>[2x]AGHMKEIKEITKKDVQDAEIYLYGSVVEG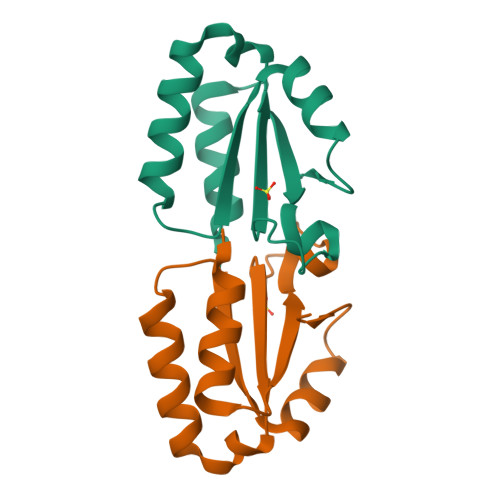DYSIGLSDIDVAIVSDVFEDRNRKLEFFGKITKKFFDSPFEFHILTKKEWKMSKRFIRKYRRLDLIT> GAMAHGIPSQGKVTITVDEYSSNPTQAFTHYNINQSRFQPPHVHMVDPIPYDTPKPAGHTRFVCISDTHSRTDGIQMPYGDILLHTGDFTELGLPSEVKKFNDWLGNLPY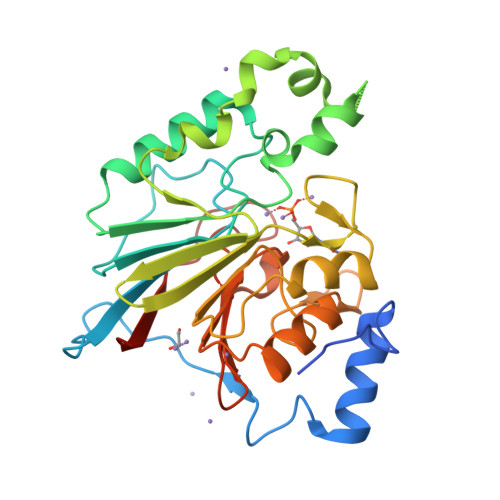EYKIVIAGNHELTFDKEFMADLVKQDYYRFPSVSKLKPEDFDNVQSLLTNSIYLQDSEVTVKGFRIYGAPWTPWFNGWGFNLPRGQSLLDKWNLIPEGTDILMTHGPPLGFRDWVPKELQRVGCVELLNTVQRRVRPKLHVFGGIHEGYGTMTDGYTTYINASTCTVSFQPTNPPIIFDLPNPQGS>SNADNALTGIELYKAKKYEQAMTHLMTPDAQKNPAAQNLIGYLYDKGLG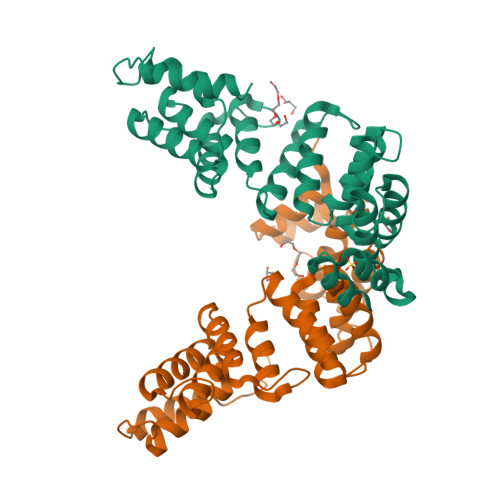VEKNAEIANQWYLKAAEQGFAKAQFNLGLSYEKGTGISKNMVEAVKWYRKAAEQNHAKAEMKMGYLTVEGIGTQKNYKEALQWYRRAAEHGDNRAYADIGLFYDQGNGVKKDPNRAVQYYIMGAEKGDGEAQLFLADCYAKASGIPYDADRALYWYKESAKNGNITAMKVLSGIYKLGQLGIEKNPEKSRHWLEMAKQKEAQP[2x]> MSFVITNPEALTVAATEVRRIRDRAIQSDAQV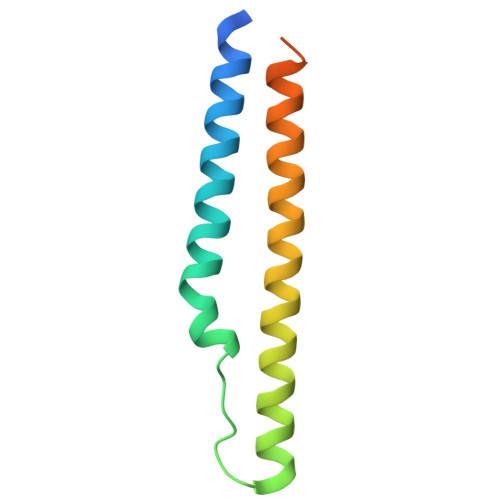APMTTAVRPPAADLVSEKAATFLVEYARKYRQTIAAAAVVLEEFAHALTTGADKYATAEADNIKTFS> ITGTSTVGVGRGVLGDQKNINTTYSTYYYLQDNTRGNGIFTYDAKYRTTLPGSLWADADNQFFASYDAPAVDAHYYAGVTYDYYKNVHNRLSYDGNNAAIRSSVHYSQGYNNAFWNGSQMVYGDGDGQTFIPLSGGIDVVAHELTHAVTDYTAGLIYQNESGAINEAISDIFGTLVEFYANKNPDWEIGEDVYTPGISGDSLRSMSDPAKYGDPDHYSKRYTGTQDNGGVHINSGIINKAAYLISQGGTHYGVSVVGI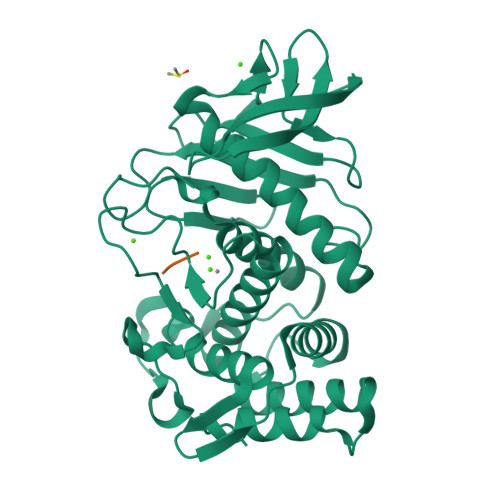GRDKLGKIFYRALTQYLTPTSNFSQLRAAAVQSATDLYGSTSQEVASVKQAFDAVGVK;> IIG> SMFLQRPKPYSDESLESFFIRVANKNGYGDVHRFLEATKRFLQDIDHNGYQTFPTDITRINPYSAKNSSSARTASFLKLAQLTFNEPPELLGLAINRTNMKYSPSTSAVVRGAEVFPRSLLRTHSIPCCPLCLRENGYASYLWHFQGYEYCHSHNVPLITTCSCGKEFDYRVSGLKGICCKCKEPITLTSRENGHEAACTVSNWLAGHESKPLPNLPKSYRWGLVHWWMGIKDSEFDHFSFVQFFSNWPRSFHSIIEDEVEFNLEHAVVSTSELRLKDLLGRLFFGSIRLPERNLQHNIILGELLCYLENRLWQDKGLIANLKMNALEATVMLNCSLDQIASMVEQRILKPNRKSKPNSPLDVTDYLFHFGDIFCLWLAEFQSDEFNRSFYVSRW

Recently, bioinformatics analyses have revealed the presence of CRISPR–Cas loci in bacterial Tn7-like transposons, thereby implicating a functional relationship between RNA-guided DNA targeting and transposition, with the latter representing a new role unrelated to host defense. Support for this concept has emerged from recent functional studies on type I-F and type V-K effectors involved in sequence-specific DNA transposition, thereby significantly broadening the potential biological applications of CRISPR–Cas technology. To complement the available functional studies, our efforts have focused on structural studies of the Vibrio cholerae Tn6677 multi-subunit type I-F CascadecrRNA–TniQ complex, whereby transposition subunit TniQ initiates DNA transposition with the eventual help of other transposition-associated proteins TnsA, TnsB and TnsC in the gene cluster. Here we report cryo-EM structures of a V. cholerae type I-F CascadecrRNA in complex with transposition subunit TniQ before (binary CascadecrRNA–TniQ) and after (ternary CascadecrRNA–TniQ–dsDNA) target double-stranded DNA (dsDNA) binding at an average resolution of 2.9 Å and 3.2 Å, respectively.

We also determined the crystal structure of apo-TniQ at 2.1 Å resolution, demonstrating that TniQ forms a head-to-tail dimer with a dimeric interface of 1931 Å2. The dimer result was confirmed by SEC-MALS in solution. Superposition of the TniQ dimer in the cryo-EM structure of ternary CascadecrRNA–TniQ–dsDNA complex (in color) with the crystal structure of the apo-form (in grey) reveals minimal conformational changes with an RMSD of 1.19 Å; the loop interacting with Cas6 becomes ordered and the helix interacting with Cas7.1 undergoes slight movement (circled in green).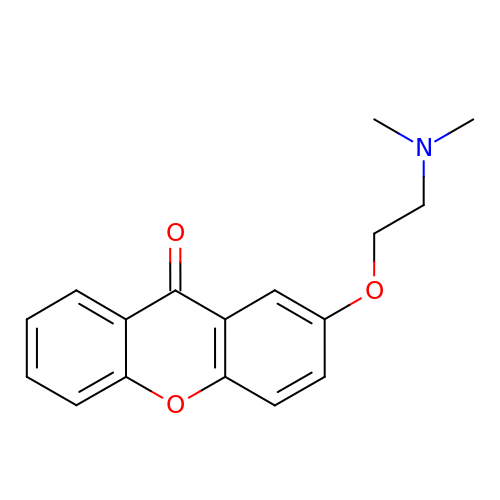2-[2-(dimethylamino)ethoxy]xanthen-9-one | C17 H17 N O3 | ZMRHVXPPMFZZHV-UHFFFAOYSA-N> KERQKVVEQMEHEMKEAAKALDFERAAELRDLLLELK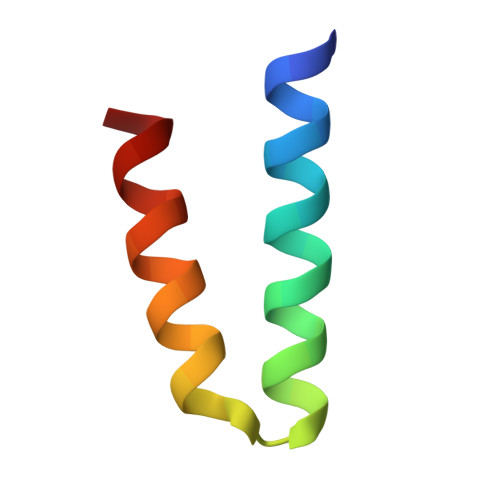A>[2x]TEDERRELEKVARKAIEAAREGNTDEVREQLQRALEIARESGSEEAFKLALEVVRRVAEVAARAGNVEAVKEALRVALEIVKEAMELIKDPEAIVRLALEAVRVVAEVAARAGAVEAVKVALRVALEIAKIAGTEEAVRLALEVVKRVSDIAKKAGNEDAVKEAEEVRKKIEEESGGSGSHHWGSTHHHHHH

We set out to design proteins that can switch between two well-defined and fully structured conformations. We reasoned that these goals could be collectively achieved with a “hinge”-like design in which two rigid domains move relative to each other while remaining individually folded. The hinge amplifies small local structural and chemical changes to achieve large global changes while the chemical environment for most residues remains similar throughout the conformational change, avoiding the need for global unfolding. Designing one of the resulting conformations to bind to a target effector couples the conformational equilibrium with target binding.

The backbone conformation of the DHR serves as the first conformational state of our hinge protein (“state X”). We solved crystal structures for two designs, cs207 and cs074. For design cs207, crystals were obtained from two separate crystallization screens: one screen for the hinge alone, and one screen for the hinge in complex with the target peptide. In the absence of peptide the experimental structure agrees well with the state X design model, and the structure of the hinge-peptide complex agrees well with the state Y design model. The crystal structures of hinge cs207 in both designed states demonstrate the accuracy with which two very different conformational states of the same protein can now be designed.>MAKRVAIVGAGVSGLASIKCCLEEGLEPTCFERSDDLGGLWRFTEHVEEGRASLYKSVVSNSCKEMSCYSDFPFPEDYPNYVPNSQFLEYLKMYANRFNLLKHIQFKTKVCSVTKCPDFTVTGQWEVVTQHEGKQESAIFDAVMVCTGFLTDPYLPLDSFPGINTFKGQYFHSRQYKHPDIFKDKRVLVVGMGNSGTDIAVEASHLAKKVFLSTTGGAWVMSRVFDSGYPWDMVFTTRFQNMLRNSLPTPIVTWLMARKMNSWFNHANYGLVPEDRTQLREPVLNDELPGCIITGKVLIKPSIKEVKENSVIFNNTPKEEPIDIIVFATGYTFAFPFLDESVVKVENGQASLYKYIFPAHLPKPTLAVIGLIKPLGSIIPTGETQARWAVRVLKGINKLPPQSVMIEEVNARKENKPSGFGLCYCKALQSDYITYIDELLTYINAKPNLLSMLLTDPRLALTIFFGPCTPYQFRLTGPGKWEGARNAILTQWDRTFKVTKTRIVQESPSPFASLLKLLSLPVLLLALLLMC[4x]

Mammals rely on the oxidative flavin-containing monooxygenases (FMOs) to detoxify numerous and potentially deleterious xenobiotics; this activity extends to many drugs, giving FMOs high pharmacological relevance. As such, we hereby reconstructed the mammalian ancestral protein sequences of both FMO1 and FMO4, denoted as ancestral flavin-containing monooxygenase (AncFMO)1 and AncFMO4, respectively. AncFMO1, sharing 89.5% sequence identity with human FMO1, was successfully expressed as a functional enzyme. It displayed typical FMO activities as demonstrated by oxygenating benzydamine, tamoxifen, and thioanisole, drug-related compounds known to be also accepted by human FMO1, and both NADH and NADPH cofactors could act as electron donors, a feature only described for the FMO1 paralogs.

We were able to successfully crystallize AncFMO1 and to solve its structure at 3.0 Å resolution. The asymmetric unit consisted of two dimers, and the dimerization observed for AncFMO1 is the same as for the dimers documented by the other AncFMO crystal structures. Alongside the well-conserved NAD(P)H- and FAD-binding domains, known as the paired Rossmann fold, AncFMO1 includes a large 80-residue insertion, two small α-helical triads that form the hydrophobic ridge that embeds into the phospholipid bilayer, and a large transmembrane C-terminal helix that drills into the membrane. The oxidized coenzyme, NADP+, was successfully bound in the crystal structure and two glycerol molecules were found located near/at the active site. AncFMO1 possesses a phenylalanine and a leucine at positions 149 and 150, respectively, creating a hydrophobic and wider pocket at the base of the active site. Furthermore, with Leu150 not being able to create hydrogen bonds, Lys373 is not tied down and can extend outward, toward a glycerol molecule situated below the diphosphate moiety of the NADP+, thereby further enlarging the active site. While the other AncFMOs crystal structures portray the 2’-phosphate to be extended out into the solvent, in the AncFMO1 crystal structure, the 2’-phosphate is tucked inside the NADP+ binding domain. More specifically, the 2’-phosphate establishes hydrogen bonds with the side chains of Arg280 and Thr214, and the peptide of Met192. Nonetheless, unlike the other characterized crystal structures that conveyed closed active-site cavities, AncFMO1 exhibits a significantly porous active site. First, the residue changes at the base of the active site (Leu150, Phe149, and Lys373,) create a hole in the vestibule and a leaky cavity. This is in turn emphasized by a large loop (residues 416–425) that further expands the substrate entry point.>[4x]GPGRAKFKHQGLVADLLPNIRVMQGVGHFMFNYYSEGKKFPHRIYCIVTLLLLLLQYGMMAVNLMMESDDVDDLTANTITMLFFLHPIVKMIYFPVRSKIFYKTLAIWNNPNSHPLFAESNARFHALAITKMRRLLFC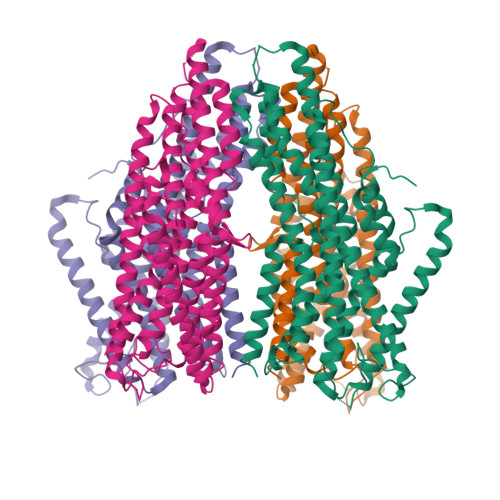VAGATIFSVISWTGITFIEDSVKRITDPETNETTIIPIPRLMIRTFYPFNAMSGAGHVFALIYQFYYLVISMAVSNSLDVLFCSWLLFACEQLQHLKAIMKPLMELSATLDTVVPNSGELFKAGSADHLRESQGVQPSGNGDNVLDVDLRGIYSNRQDFTATFRPTAGTTFNGGVGPNGLTKKQEMLVRSAIKYWVERHKHVVRLVTAVGDAYGVALLLHMLTTTITLTLLAYQATKVNGVNVYAATVIGYLLYTLGQVFLFCIFGNRLIEESSSVMEAAYSCHWYDGSEEAKTFVQIVCQQCQKAMSISGAKFFTVSLDLFASVLGAVVTYFMVLVQLK>[2x]MDIEDERLEELDERAESVVQLGDEVVLGTAEQELKQAPGVSIITAEDIRKRPPVNDLSEIIRTMPGVNLTGNSSSGQRGNNRQIDIRGMGPENTLILVDGKPVSSRNSVRYGWRGERDTRGDSNWVPPEEVERIEVLRGPAAARYGSGAAGGVVNIITKRPTDRLRGSMTVFTNIPESS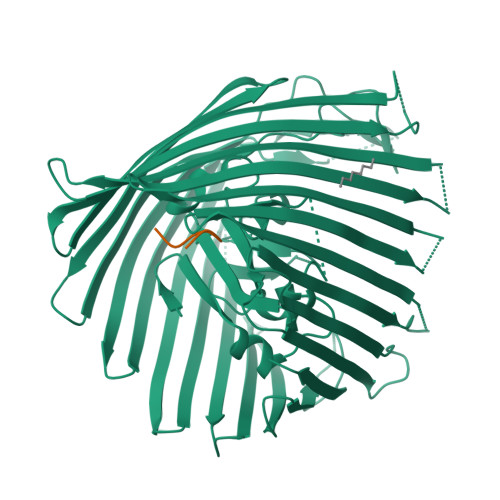KDGATRRANFSLSGPLTEALSFRAYGSANKTDSDDTDINLGHTVNPSRTVAGREGVRNRDLSGMLSWQVTPDQVVDFEAGFSRQGNIYAGDTQNNNGTANTQGLADDGAETNRMYRENYAITHNGTWSFGTSRFVAQYDSTRNNRLEEGLAGSVEGQIGADRSFSASKLENYRLSGELNLPLHALFEQVLTVGAEWNKETLNDPSSLKQGFVGSDSLPGTPAAGSRSPKSKAEIRALYVEDNIELRPGTMLTPGLRLDDHSDFGLNWSPSLNASQTLGEYFTVKAGIARAFKAPNLYQSNPNYLLYTRGNGCPIQTSSGGCYLVGNENLDAETSVNKELGIEFRRDGWVAGLTYFRNDYKNKIVAPLDVMGQTGTGNNILQWSNAKKAVVEGLEGNLLVPLHEDLSWSTNLTYMLQSKDKDTGNPLSVIPEYTLNSTLDWQASERLSTQLTSTIYGRQEPPKHGTSRNTPVVSRKEVGTYGIWGVSAGYTFSENLSVRGGVSNLFDKRLYRQGNSFDAGAATYNEPGRAYYVSMTTSFLSHHHHHH>[2x]AMGSDVVDPDIFNRDPRDHYDLLQRLGGGTYGEVFKARDKVSGDLVALKMVKMEPDDDVSTLQKEILILKTCRHANIVAYHGSYLWLQKLWICMEFCGAGSLQDIYQVTGSLSELQISYVCREVLQGLAYLHSQKKIHRDIKGANILINDAGEVRLADFG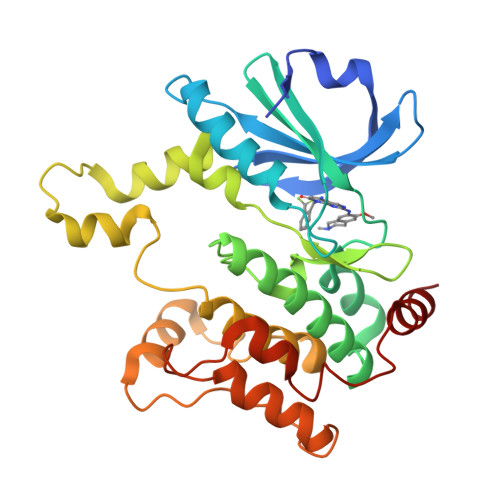ISAQIGAELARRLEFIGTPYWMAPEVAAVALKGGYNELCDIWSLGITAIELAELQPPLFDVHPLRVLFLMTKSGYQPPRLKEKGKWSAAFHNFIKVTLTKSPKKRPSATKMLSHQLVSQPGLNRGLILDLLDKLKN>DALKPEDKVKFRQASYTTMAWNMGKIKAMVVDGTMPFSQTQVSAAANVIAAIANSGMGALYSPDTLGVVGFKKSRLKENFFQEQDEVRKIATNFVEQANKLAEVAAMGDKDEIKAQFGEVGKACKACHEKFREEE[4x]

Thermophilic Hydrogenophilus thermoluteolus cytochrome c′ (PHCP) exhibits higher thermal stability than a mesophilic counterpart, Allochromatium vinosum cytochrome c′ (AVCP), which has a homo‐dimeric structure and ligand‐binding ability. A spectroscopic study clearly showed that some ligands were bound to the PHCP protein. It is concluded that the dimeric PHCP from the thermophile is effectively stabilized through heme‐related and subunit–subunit interactions with conservation of the ligand‐binding ability.

To understand the thermal stability mechanism and ligand‐binding ability of the thermally stable PHCP protein, the crystal structure of PHCP was first determined. It formed a homo‐dimeric structure, the main chain root mean square deviation (rmsd) value between PHCP and AVCP being 0.65 Å. In the PHCP structure, six specific residues appeared to strengthen the heme‐related and subunit–subunit interactions, which were not conserved in the AVCP structure. PHCP variants having altered subunit–subunit interactions were more severely destabilized than ones having altered heme‐related interactions. The PHCP structure further revealed a ligand‐binding channel and a penta‐coordinated heme, as observed in the AVCP protein.> AMYSTNAYAELAGPPKIFCKSVSKDPDFRLKQIDYVIPVQQDRSICMNNPLLDISDGFFTYIHYEGINSCKKSDSFKVLLSHGEIVDRGDYRPSLYLLSSHYHPYSMQVINCVPVTCNQSSFVFCHISNNTKTLDNSDYSSDEYYITYFNGIDRPKTKKIPINNMTADNRYIHFTFSGGGGVCLGEEFIIPVTTVINTDVFTHDYCESFNCSVQTGKSLKEICSESLRSPTNSSRYNLNGIMIISQNNMTDFKIQLNGITYNKLSFGSPGRLSKTLGQVLYYQSSMSWDTYLKAGFVEKWKPFTPNWMNNTVISRPNQGNCPRYHKCPEICYGGTYNDIAPLDLGKDMYVSVILDSDQLAENPEITVFNSTTILYKERVS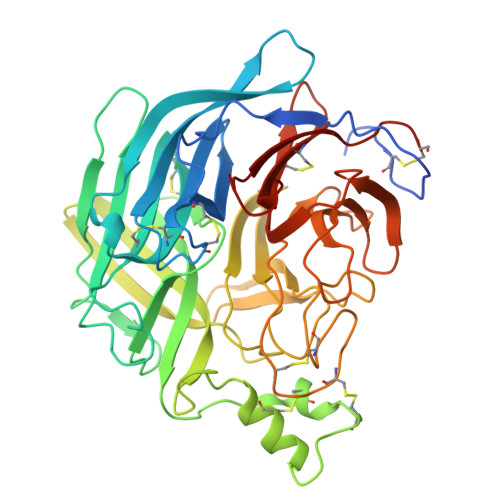KDELNTRSTTTSCFLFLDEPWCISVLETNRFNGKSIRPEIYSYKIPKYC>GCGGDLWRQRLWIVDDRTAYRPHANGVIWIWE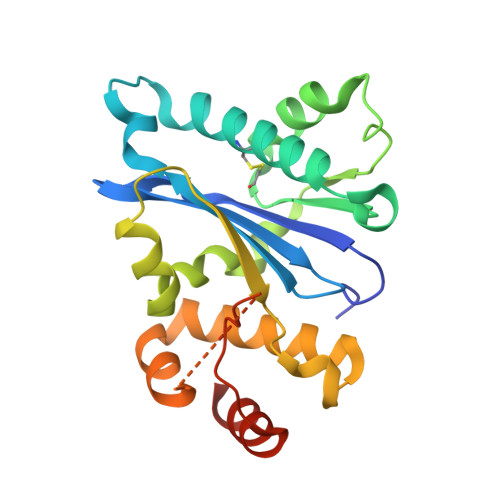TSTGRLFVKIVHRTTWAGQTRRAQLAKWKCAEHVLTMLRSQPTEELPRGIVLAQTASMDPLKTLLAGTEYAKIPVRAGAAAMPLQALMALPEIRDRTQTARSSELSIWSGYADWLEHVPVWIASARFLLLLHALDRAPERVLQLVWPQRSADEESAGSATPWLWPALPETDWRRLELELQSLVPVR[2x]>MKIGANYTPSQGWFHSWLDLDIDATRRDFEGIAQLGLDHVRLFPLWPLLQPNRGLVRPRALDDVVSVVRAAGEFDLEVTVDALNGHLSSYDFLPPWVITWHTSNLFTDPLVKAGQTDLISQLATRLREEPNATGMTVGNEFPQYAALAPGHHHPTRSECTVDDAQTWLETMLGTMRDQWPDGRFWFGFDDDLWFVDDHPFTPRHAVTQGSATTVHSWVFAQVGPRFGEGHPALTWFPRYLLELARAWSHDPERPLWLQEVGAPRTHVPDSSSAAFMTTTMASLTSTPGLEAITWWCSHDVSRDLLDFPELEYSLGLFTNDGKPKPEALALSDMLPDLHNAQPQHQLDEPLEFSANWDTGAGRSVCSPMGDLFAQWVDQAEQTGRAPRLALRPTPGLTDREALASARAHSAHHHHHH[4x]

The gram-positive bacterium Cutibacterium acnes (formerly Propionibacterium acnes) belongs to the phylum Actinobacteria, and is one of the major inhabitants of the sebaceous follicles of the human skin. In this work, we propose a degradation pathway for the cytoplasmic path of host N-glycans by C. acnes, as well as a detailed structural and functional characterization of the exo-β-1,4-mannosidase, a member of glycoside hydrolase family 5 subfamily 18 (GH5_18), that catalyzes hydrolysis of the β-1,4-glycosidic bond between the second N-acetylglucosamine and the first mannose residue in the canonical eukaryotic N-glycan core. The amino-acid sequences of exo-acting β-mannosidases (EC 3.2.1.25) are found in any of the three GH families 1, 2 and 5, which belong to the GH-A clan that features the (β/α)8 TIM-barrel fold. These enzymes follow a retaining reaction mechanism according to the classical Koshland double-displacement mechanism where two conserved glutamate residues act as acid/base catalyst and nucleophile.

The crystal structure of CaMan5_18 was determined and refined in the unliganded state at a final resolution of 1.8 Å. The crystals belong to space group P21 with four molecules in the asymmetric unit, and an approximate solvent content of 50%. The overall structure displays the, for GH5 enzymes typical, (β/α)8 TIM-barrel fold. The enzyme was co-crystallized with mannose, however, no clear density for the sugar could be identified. Furthermore, we were unsuccessful in capturing a complex of CaMan5_18 with mannose, probably because a disordered MOPS molecule is present in the active site of the crystal structure. Although the experimental data do not show bound ligand in the active site, we can derive from close homologs that Glu140 is acting as the acid/base catalyst and Glu259 as a nucleophile. The conformation of Glu140 is supported by interactions with His215, and the neighboring Asn139 is kept in position through a possible hydrogen bond with Arg41. The orientation of the catalytic nucleophile Glu259 can be stabilized through interactions with Arg41 and Trp217. The enzyme is present as a two-fold symmetrical homodimer in the crystal, featuring an extensive dimer interface generated by five loop regions: L1 (residues 46–57), L2 (residues 89–92), L3 (residues 98–102), L4 (residues 152–156), and L5 (residues 299–314), where especially L2 and L3 shape and stabilize the active site (inset). The C-terminus in our CaMan5_18 structure (residues 396–408) is flexible and lacks interpretable electron density.5-{4-[3-(4-{[(2R)-2-hydroxy-3,3-dimethylbutyl]oxy}-3-methylphenyl)pentan-3-yl]-2-methylphenoxy}pentanoic acid | C30 H44 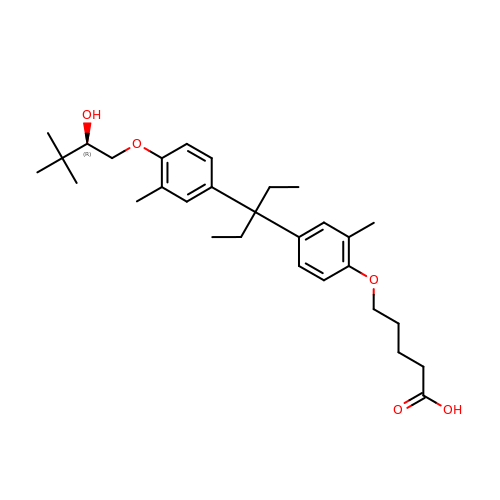O5 | CWFBRPYCPUENQV-MHZLTWQESA-N>[10x]MKINVSRPLQFLQWSSYIVVAFLIQLLIILPLSILIYHDFYLRLLPADSSNVVPLNTFNILNGVQFGTKFFQSIKSIPVGTDLPQTIDNGLSQLIPMRDNMEYKLDLNLQLY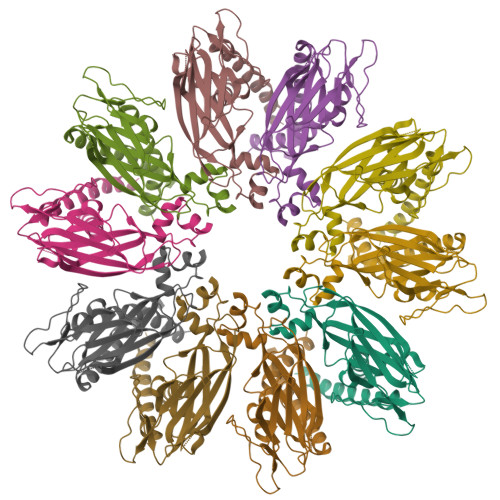CQSKTDHLNLDNLLIDVYRGPGPLLGAPGGSNSKDEKIFHTSRPIVCLALTDSMSPQEIEQLGPSRLDVYDEEWLNTIRIEDKISLESSYETISVFLKTEIAQRNLIIHPESGIKFRMNFEQGLRNLMLRKRFLSYIIGISIFHCIICVLFFITGCTAFIFVRKGQEKSKKHS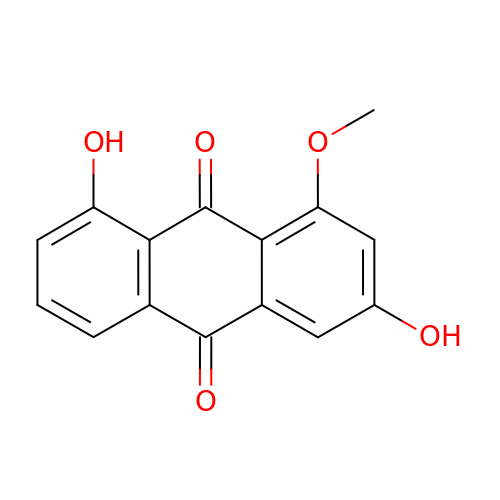1-methoxy-3,8-bis(oxidanyl)anthracene-9,10-dione | C15 H10 O5 | MKPXKUVNBNOJOI-UHFFFAOYSA-N> MQSKVLLAVALWLCVETRAASVGLPSVSLDLPRLSIQKDILTIKANTTLQITCRGQRDLDWLWPNNQSGSEQRVEVTECSDGLFCKTLTIPKVIGNDTGAYKCFYRETDLASVIYVYVQDYRSPFIASVSDQHGVVYITENKNKTVVIPCLGSISNLNVSLCARYPEKRFVPDGNRISWDSKKGFTIPSYMISYAGMVFCEAKINDESYQSIMYIVVVVGYRIYDVVLSPSHGIELSVGEKLVLNCTARTELNVGIDFNWEYPSSKHQHKKLVNRDLKTQSGSEMKKFLSTLTIDGVTRSDQGLYTCAASSGLMTKKNSTFVRVHEKPFVAFGSGMESLVEATVGERVRIPAKYLGYPPPEIKWYKNGIPLESNHTIKAGHVLTIMEVSERDTGNYTVILTNPISKEKQSHVVSLVVYVPPQIGEKSLISPVDSYQYGTTQTLTCTVYAIPPPHHIHWYWQLEEECANEPSQAVSVTNPYPCEEWRSVEDFQGGNKIEVNKNQFALIEGKNKTVSTLVIQAANVSALYKCEAVNKVGRGERVISFHVTRGPEITLQPDMQPTEQESVSLWCTADRSTFENLTWYKLGPQPLPIHVGELPTPVCK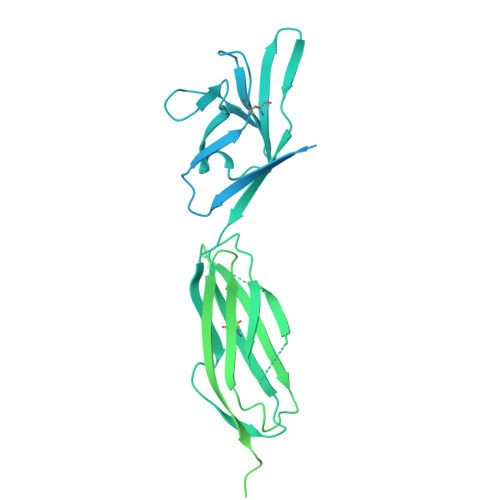NLDTLWKLNATMFSNSTNDILIMELKNASLQDQGDYVCLAQDRKTKKRHCVVRQLTVLERVAPTITGNLENQTTSIGESIEVSCTASGNPPPQIMWFKDNETLVEDSGIVLKDGNRNLTIRRVRKEDEGLYTCQACSVLGCAKVEAFFIIEGAQEKTNLERTHHHHHH> MAMQTSTSSLAKQLFQMTWPMLFGVLSLMSFQLVDSAFIGQLGVLPLAAQGFTMPIQMVIIGIQVGLGIATTAVISRAIGAGKTEYAKQLGGLVIVIGGIGVALIALVLYLLRQPLLGLLGAPETVFAIIDHYWLWWLASAWTGAMLYFYYSVCRANGNTLLPGTLMMVTSVLNLILDPIFIFTFDLGIDGAAIATIIAFGVGIAIVAPKVAQRQWTSYQWQDLNISQSLTALGHIMGPAMLSQLLPPLSSMFATKLLASFGT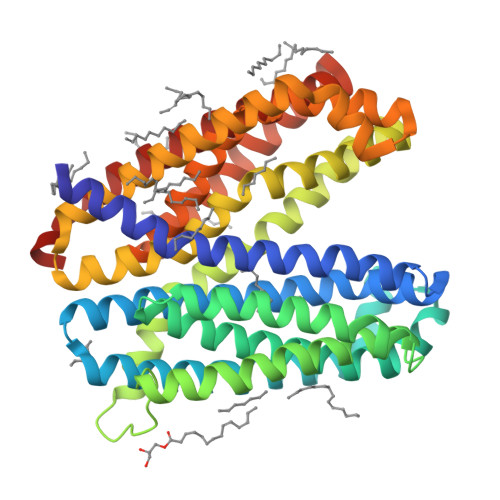AAVAAWALGSRFEFFALVAVLAMTMSLPPMIGRMLGAKEITHIRQLVRIACQFVLGFQLLIALVTYVFATPLAELMTSETEVSQILNLHLVIVPISLGALGICMLMVSVANALGKSYVALTISALRLFAFYLPCLWLGAHFYGIEGLFIGALVGNIIAGWAAWLAYQKALRSENLYFQ>[6x]MRGSHHHHHHGSMPVAGSELPRRPLPPAAQERDAEPRPPHGELQYLGQIQHILRCGVRKDDRTGTGTLSVFGMQARYSLRDEFPLLTTKRVFWKGVLEELLWFIKGSTNAKELSSKGVKIWDANGSRDFLDSLGFSTREEGDLGPVYGFQWRHFGAEYRDM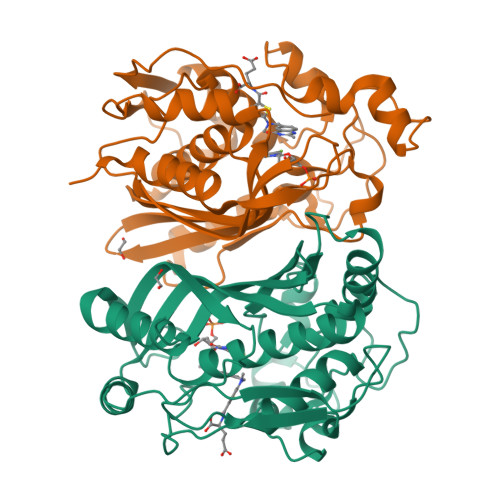ESDYSGQGVDQLQRVIDTIKTNPDDRRIIMCAWNPRDLPLMALPPCHALCQFYVVNSELSCQLYQRSGDMGLGVPFNIASYALLTYMIAHITGLKPGDFIHTLGDAHIYLNHIEPLKIQLQREPRPFPKLRILRKVEKIDDFKAEDFQIEGYNPHPTIKMEMAV> APSYPEYTREEVGRHRSPEERVWVTHGTDVFDVTDFVELHPGGPDKILLAAGGALEPFWALYAVHGEPHVLELLQQYKVGELSPDEAPAAPDAQDPFAGDPPRHPGLRVNSQKPFNAEPPAELLAERFLTPNELFFTRNHLPVPAVEPSSYRLRVDGPGGGTLSLSLAELRSRFPKHEVTATLQCAGNRRSEMSRVRPVKGLPWDIGAISTARWGGARLRDVLLHAGFPEELQGEWHVCFEGLDADPGGAPYGASIPYGRALSPAADVLLAYEMNGTELPRDHGFPVRVVVPGVVGARSVKWLRRVAVSPDESPSHWQQNDNKGFSPCVDWDTVDYRTAPAIQELPVQSAVTQPRPGAAVPPGE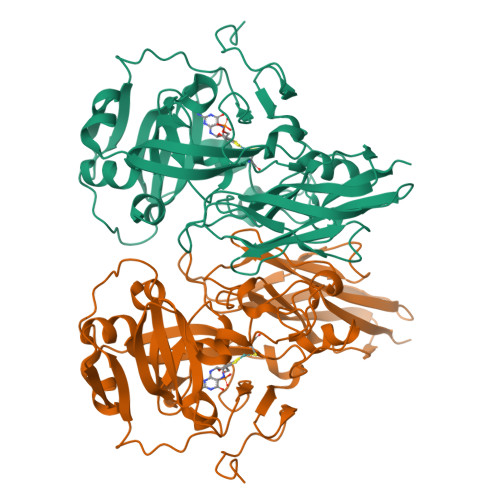LTVKGYAWSGGGREVVRVDVSLDGGRTWKVARLMGDKAPPGRAWAWALWELTVPVEAGTELEIVCKAVDSSYNVQPDSVAPIWNLMGMLSTAWHRVRVSVQD>[2x]MLESKLKAPVFTATTQGDHYGEFVLEPLERGFGVTLGNPLRRILLSSIPGTAVTSVYIEDVLHE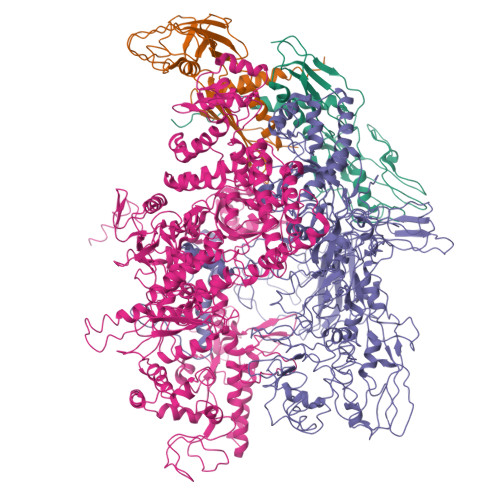FSTIPGVKEDVVEIILNLKELVVRFLDPKMASTTLILRAEGPKEVRAGDFTPSADVEIMNPDLHIATLEEGGKLYMEVRVDRGVGYVPAERHGIKDRINAIPVDAIFSPVRRVAFQVEDTRLGQRTDLDKLTLRIWTDGSVTPLEALNQAVAILKEHLNYFANPEASLLPTPEVSKGEKRESAEEDLDLPLEELGLSTRVLHSLKEEGIESVRALLALNLKDLRNIPGIGERSLEEIRQALAKKGFTLKE;> MEIKRFGRIREVIPLPPLTEIQVESYKKALQADVPPEKRENVGIQAAFKETFPIEEGDKGKGGLVLDFLEYRIGDPPFSQDECREKDLTYQAPLYARLQLIHKDTGLIKEDEVFLGHLPLMTEDGSFIINGADRVIVSQIHRSPGVYFTPDPARPGRYIASIIPLPKRGPWIDLEVEASGVVTMKVNKRKFPLVLLLRVLGYDQETLVRELSAYGDLVQGLLDEAVLAMRPEEAMVRLFTLLRPGDPPKKDKALAYLFGLLADPKRYDLGEAGRYKAEEKLGVGLSGRTLVRFEDGEFKDEVFLPTLRYLFALTAGVPGHEVDDIDHLGNRRIRTVGELMADQFRVGLARLARGVRERMVMGSPDTLTPAKLVNSRPLEAALREFFSRSQLSQFKDETNPLSSLRHKRRISALGPGGLTRERAGFDVRDVHRTHYGRICPVETPEGANIGLITSLAAYARVDALGFIRTPYRRVKNGVVTEEVVYMTASEEDRYTIAQANTPLEGDRIATDRVVARRRGEPVIVAPEEVEFMDVSPKQVFSLNTNLIPFLEHDDANRALMGSNMQTQAVPLIRAQAPVVMTGLEERVVRDSLAALYAEEDGEVVKVDGTRIAVRYEDGRLVEHPLRRYARSNQGTAFDQRPRVRVGQRVKKGDLLADGPASEEGFLALGQNVLVAIMPFDGYNFEDAIVISEELLKRDFYTSIHIERYEIEARDTKLGPERITRDIPHLSEAALRDLDEEGIVRIGAEVKPGDILVGRTSFKGEQEPSPEERLLRSIFGEKARDVKDTSLRVPPGEGGIVVGRLRLRRGDPGVELKPGVREVVRVFVAQKRKLQVGDKLANRHGNKGVVAKILPVEDMPHLPDGTPVDVILNPLGVPSRMNLGQILETHLGLAGYFLGQRYISPVFDGATEPEIKELLAEAFNLYFGKRQGEGFGVDKREKEVLARAEKLGLVSPGKSPEEQLKELFDLGKVVLYDGRTGEPFEGPIVVGQMFIMKLYHMVEDKMHARSTGPYSLITQQPLGGKAQFGGQRFGEMEVWALEAYGAAHTLQEMLTIKSDDIEGRNAAYQAIIKGEDVPEPSVPESFRVLVKELQALALDVQTLDEKDNPVDIFEGLASKR;> MKKEVRKVRIALASPEKIRSWSYGEVEKPETINYRTLKPERDGLFDERIFGPIKDYECACGKYKRQRFEGKVCERCGVEVTRSIVRRYRMGHIELATPAAHIWFVKDVPSKIGTLLDLSATELEQVLYFNKYIVLDPKGAVLDGVPVEKRQLLTDEEYGGIDARMGAEAIQELLKELDLEKLERELLEEMKHPSRARRAKARKRLEVVRAFLDSGNRPEWMILEAVPVLPPDLRPMVQVDGGRFATSDLNDLYRRLINRNNRLKKLLAQGAPEIIIRNEKRMLQEAVDAVIDNGRRGSPVTNPGSERPLRSLTDILSGKQGRFRQNLLGKRVDYSGRSVIVVGPQLKLHQCGLPKRMALELFKPFLLKKMEEKAFAPNVKAARRMLERQRDIKDEVWDALEEVIHGKVVLLNRAPTLHRLGIQAFQPVLVEGQSIQLHPLVCEAFNADFDGDQMAVHVPLSSFAQAEARIQMLSAHNLLSPASGEPLAKPSRDIILGLYYITQVRKEKKGAGMAFATPEEALAAYERGEVALNAPIVVAGRETSVGRLKFVFANPDEALLAVAHGLLDLQDVVTVRYLGRRLETSPGRILFARIVGEAVGDEKVAQELIQMDVPQEKNSLKDLVYQAFLRLGMEKTARLLDALKYYGFTLSTTSGITIGIDDAVIPEEKQRYLEEADRKLRQIEQAYEMGFLTDRERYDQVIQLWTETTEKVTQAVFKNFEENYPFNPLYVMAQSGARGNPQQIRQLCGMRGLMQKPSGETFEVPVRSSFREGLTVLEYFISSHGARKGGADTALRTADSGYLTRKLVDVAHEIVVREADCGTTNYISVPLFQMDEVTRTLRLRKRSDIESGLYGRVLAREVEALGRRLEEGRYLSLEDVHFLIKAAEAGEVREVPVRSPLTCQTRYGVCQKCYGYDLSMARPVSIGEAVGVVAAESIGEPGTQLTMRTFHTGGVAVGTDITQGLPRVIELFEARRPKAKAVISEIDGVVRIEEGEDRLSVFVESEGFSKEYKLPKDARLLVKDGDYVEAGQPLTRGAIDPHQLLEAKGPEAVERYLVDEIQKVYRAQGVKLHDKHIEIVVRQMLKYVEVTDPGDSRLLEGQVLEKWDVEALNERLIAEGKVPVAWKPLLMGVTKSALSTKSWLSAASFQNTTHVLTEAAIAGKKDELIGLKENVILGRLIPAGTGSDFVRFTQVVDQRTLKAIEEARKEAVEAKEKEAPRRPVRREQPGKGL> GDAICIFRELQCLTPRGRYDIRIYPTFLHLHGKTFDYKIPYTTVLRLFLLPHKDQRQMFFVISLDPPIKQGQTRYHFLILLFSKDEDISLTLNMNEEEVEKRFEGRLTKNMSGSLYEMVSRVMKALVNRKITVPGNFQGHSGAQCITCSYKASSGLLYPLERGFI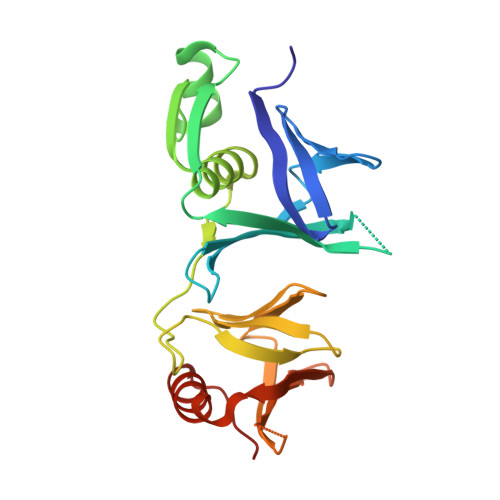YVHKPPVHIRFDEISFVNFARGTTTTRSFDFEIETKQGTQYTFSSIEREEYGKLFDFVNAKKLNIKNRGL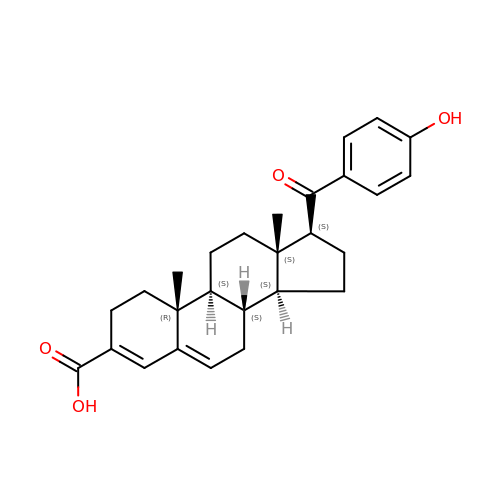(8alpha,10alpha,13alpha,17beta)-17-[(4-hydroxyphenyl)carbonyl]androsta-3,5-diene-3-carboxylic acid | C27 H32 O4 | RPNNXCYIESWDSC-JRZBRKEGSA-N>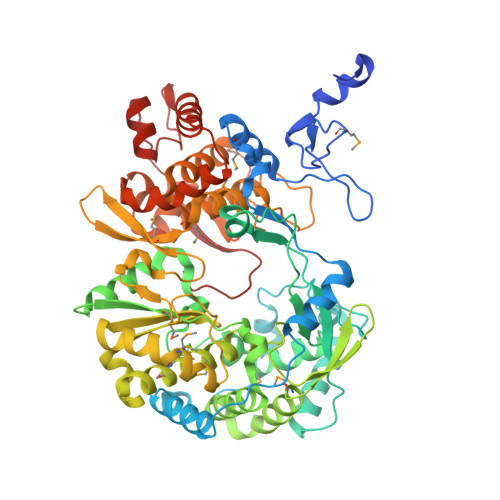 AYLKLKDFIEEEEKKPRVKDTVIREHNKWILKKIRFQGNLNTKKMLNPGKLSEQLDREGRKRNIYNHQIGTIMSSAGIRLEKLPIVRAQTDTKTFHEAIRDKIDKSENRQNPELHNKLLEIFHTIAQPTLKHTYGEVTWEQLEAGVNRKGAAGFLEKKNIGEVLDSEKHLVEQLVRDLKAGRKIKYYETAIPKNEKRDVSDDWQAGDLVVEKRPRVIQYPEAKTRLAITKVMYNWVKQQPVVIPGYEGKTPLFNIFDKVRKEWDSFNEPVAVSFDTKAWDTQVTSKDLQLIGEIQKYYYKKEWHKFIDTITDHMTEVPVITADGEVYIRNGQRGSGQPDTSAGNSMLNVLTMMYAFCESTGVPYKSFNRVARIHVCGDDGFLITEKGLGLKFANKGMQILHEAGKPQKITEGEKMKVAYRFEDIEFCSHTPVPVRWSDNTSSHMAGRDTAVILSKMATRLDSSGERGTTAYEKAVAFSFLLMYSWNPLVRRICLLVLSQQPETDPSKHATYYYKGDPIGAYKDVIGRNLSELKRTGFEKLANLNLSLSTLGVWTKHTSKRIIQDCVAIGKEEGNWLVKPDRLISSKTGHLYIPDKGFTLQGKHYEQLQL N-hydroxy-N~2~-[(2-phenylethyl)sulfonyl]glycinamide 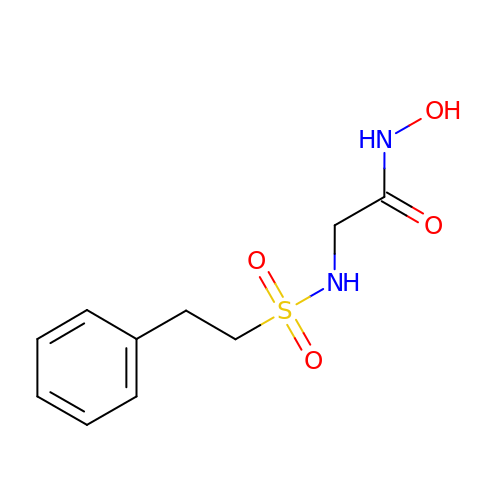| C10 H14 N2 O4 S | CWDYQHCEZVYJNX-UHFFFAOYSA-N N-(3-methylbenzene-1-carbonyl)glycine 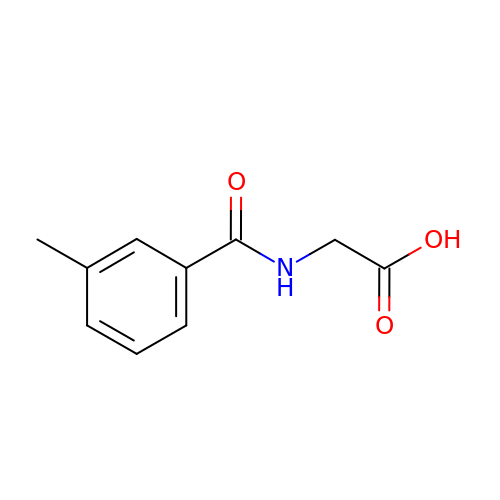| C10 H11 N O3 | YKAKNMHEIJUKEX-UHFFFAOYSA-N> DEASGIGPEEHFPEVPEIEPMGPVCPFRCQCHLRVVQCSDLGLEKVPKDLPPDTALLDLQNNKITEIKDGDFKNLKNLHTLILINNKISKISPGAFAPLVKLERLYLSKNQLKELPEKMPKTLQELRVHENEITKVRKSVFNGLNQMIVVELGTNPLKSSGIENGAFQGMKKLSYIRIADTNITTIPQGLPPSLTELHLDGNKITKVDAASLKGLNNLAKLGLSFNSISAVDNGS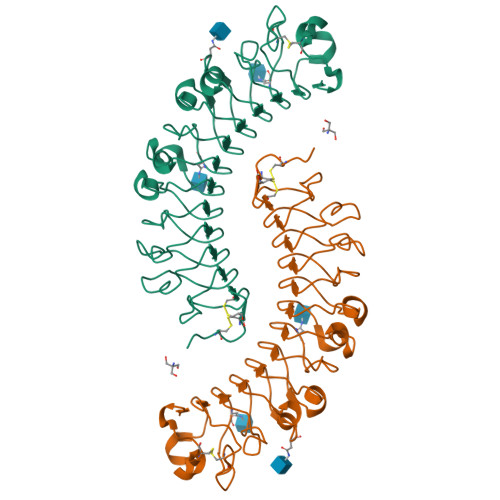LANTPHLRELHLNNNKLVKVPGGLADHKYIQVVYLHNNNISAIGSNDFCPPGYNTKKASYSGVSLFSNPVQYWEIQPSTFRCVYVRAAVQLGNYK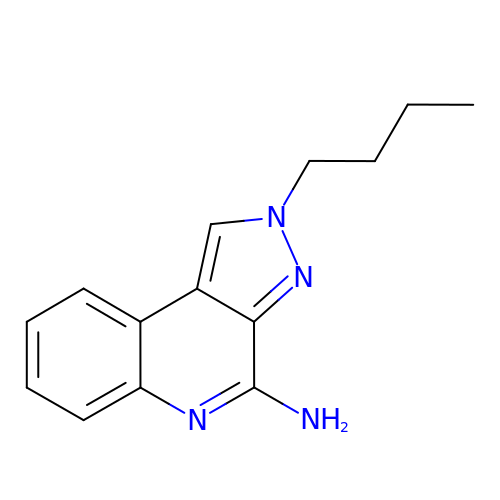2-butyl-2H-pyrazolo[3,4-c]quinolin-4-amine | C14 H16 N4 | BRUVQRFMAMBUDN-UHFFFAOYSA-N> RGSHMLEMIIKPRVRGFICVTAHPTGCEANVKKQIDYVTTEGPIANGPKRVLVIGASTGYGLAARITAAFGCGADTLGVFFERPGEEGKPGTSGWYNSAAFH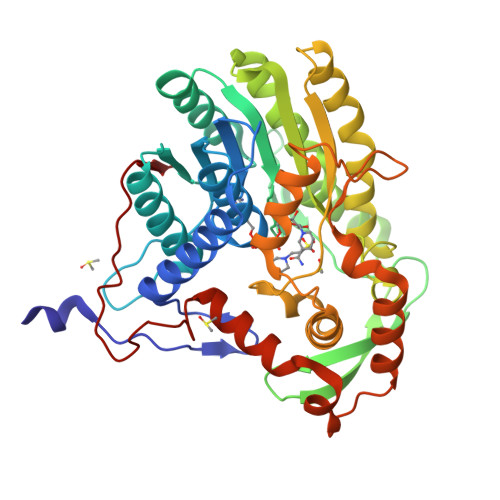KFAAQKGLYAKSINGDAFSDEIKQLTIDAIKQDLGQVDQVIYSLASPRRTHPKTGEVFNSALKPIGNAVNLRGLDTDKEVIKESVLQPATQSEIDSTVAVMGGEDWQMWIDALLDAGVLAEGAQTTAFTYLGEKITHDIYWNGSIGAAKKDLDQKVLAIRESLAAHGGGDARVSVLKAVVGQASSAIPMMPLYLSLLFKVMKEKGTHEGCIEQVYSLYKDSLCGDSPHMDQEGRLRADYKELDPEVQNQVQQLWDQVTNDNIYQLTDFVGYKSEFLNLFGFGIDGVDYDADVNPDVKIPNLIQG> SMADIKTGIFAKNVQKRLNRAQEKVLQKLGKA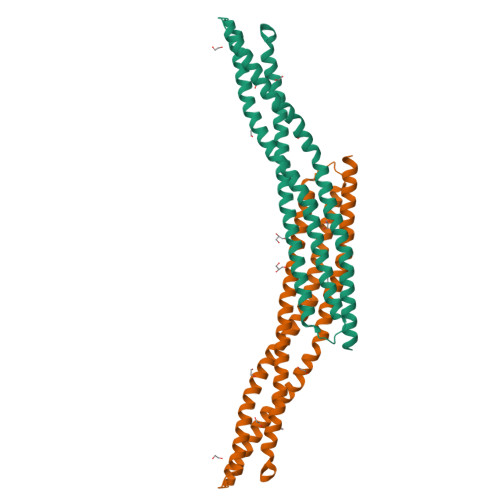DETKDEQFEEYVQNFKRQEAEGTRLQRELRGYLAAIKGMQEASMKLTESLHEVYEPDWYGREDVKMVGEKCDVLWEDFHQKLVDESLLTLDTYLGQFPDIKNRIAKRSRKLVDYDSARHHLEALQSSKRKDESRISKAEEEFQKAQKVFEEFNVDLQEELPSLWSRRVGFYVNTFKNVSSLEAKFHKEIAVLCHKLYEVMTKLGDQHADKA> MEKTFLMVKPDGVQRAFIGEIVARFEKKGFQLVGAKLMQVTPEIAGQHYAEHEEKPFFGELVDFITSGPVFAMVWQGEGVVDTARNMMGKTRPHEAAPGTIRGDFGVTVAKNIIHGSDSLESAEREIGIFFKEEELVDYSKLMNEW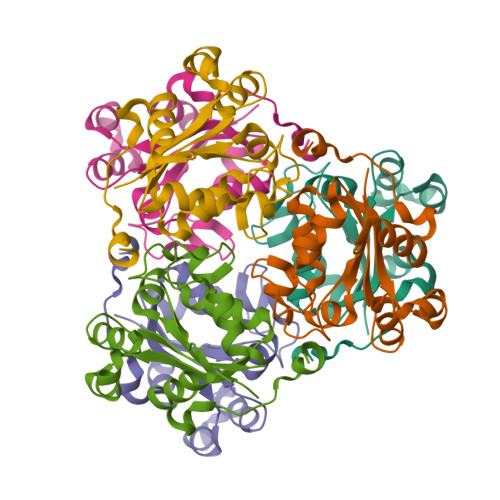IY>GSHMRQDSEVNPLQVQNSSKVLNPNVTLPANNLLYDEFFVSKESKLIEDSRNNKRKTSKIASLNPYASTKAVLTTTSSTLTSDQIVVTVPQKTFIGGVYNSTTLDNLDYTPISYPLDPITVSYSFPSDFIVDTIERPSLSSMRASVFKAMRAANFSGEQSLAFDYNIKQFSYYSELKIAFGSNVNIGKIFSIDISGSNNKIKRTTGVFAKFTQKNFTIDMDLPADGNIFKNNSDLALTNGKNPVYISSVTYGRLGIISIESNASYNEVNFALKAALTAGIVNGSLNIDSNSKKILEESDLSVYLVGGRGTDAVQVIKGFAGFSNFIVNGGQFTPEAPGVPIYFSASHASDNSVYYTTFTIDK[30x]

A recently found family of pore-forming toxins, called CDC-like proteins (CDCLs), are wide-spread in gut microbes and are a prevalent means of antibacterial antagonism. Analysis of the CDCLs belonging to the phylum Bacteroidota revealed the presence of sets of two-component CDCLs, one long CDCL (CDCLL) with four domains and one short CDCL (CDCLS) lacking the fourth C-terminal domain, that act as a bicomponent complex via a mechanism only previously observed in the mammalian complement MAC. Unlike CDCs, the CDCLs require proteolytic activation with both components containing a proteolytically cleavable activation loop critical to the regulation of pore formation. Here, we present the crystal structure of a proteolytically activated CDCLL and cryo–electron microscopy (cryo-EM) structures of a prepore-like intermediate and the transmembrane pore.

(A) The cryo-EM map at 3.13-Å resolution of the prepore-like structure from focused refinement with C30 symmetry, revealing a circular oligomer with a pore inner diameter of 164 Å and a height of 59 Å. We built an atomic model of the full prepore-like oligomer into the cryo-EM map, which consists of 30 EaCDCLS subunits, each lacking the activation loop and preceding N-terminal region. A comparison of the EaCDCLS protomer in the prepore state with the crystal structure of the monomeric proform of EaCDCLS reveals that while the α-HBs remain in their helical state, the β5 strand of the core D3 β sheet has undergone a complete β-to-α transition to create the HTH motif as observed in the membrane-inserted form of CDCs. This HTH forms a small α barrel within the interior of the circular oligomer. Thus, loss of the activation loop and corresponding β0 strand, together with the transition of β5, has allowed for the β4 and β1 strands of the core β sheet to form oligomeric contacts between adjacent subunits. This corresponds with the canonical oligomeric rearrangement and interactions observed in CDCs. Comparison of the core β sheet between monomeric EaCDCLS and the prepore-like structure also reveals the loss of the twist observed in the monomeric state, with a slight rotation and straightening of the β1-β4 strands. Therefore, we hypothesize that the stacked rings are “prepore-like” structures composed of act-EaCDCLS protein alone, similar to the circular prepore intermediate observed in CDCs. However, any putative physiological prepores would be expected to be composed of 1 EaCDCLL molecule and 29 EaCDCLS molecules, similar to the transmembrane pore, but such a short-lived intermediate would not been captured here because of the long incubation time of the experiment.>HHHHHHGSERTGTQPLGVQGLTEEQRMMIRELMDAQMKTFDTTFSHFKNFRLPGVLSSGCELPESLQAPSREEAAKWSQVRKDLCSLKVSLQLRGEDGSVWNYKPPADSGGKEIFSLLPHMADMSTYMFKGIISFAKVISYFRDLPIEDQISLLKGAAFELCQLRFNTVFNAETGTWECGRLSYCLEDTAGGFQQLLLEPMLKFHYMLKKLQLHEEEYVLMQAISLFSPDRPGVLQHRVVDQLQEQFAITLKSYIECNRPQPAHRFLFLKIMAMLTELRSINAQHTQRLLRIQDIHPFATPLMQELFGITGSSGGSGGSSHSSLTERHKILHRLLQEGSPSDITTLSVEPD[2x]

PXR is a nuclear receptor that can be activated by diverse compounds to elevate metabolism, negatively impacting drug efficacy and safety. As a xenobiotic sensor, PXR is activated by structurally diverse compounds and plays a major role in drug metabolism and drug-drug interactions by regulating transcription of genes encoding drug metabolizing enzymes, drug conjugating enzymes, and drug transporters. Here, we report structurally related PXR-selective agonists and antagonists and their corresponding co-crystal structures to describe mechanisms of antagonism and selectivity. Structural and computational approaches show that antagonists induce PXR conformational changes incompatible with transcriptional coactivator recruitment.

It should be noted that SJPYT-278 is a racemic mixture, where the (S) and (R) enantiomers were individually synthesized as SJPYT-312 and SJPYT-313, respectively. The electron density in PXR LBD complexed with the racemic SJPYT-278 mixture indicates the presence of both (R) and (S) enantiomers, likely because they have similar PXR LBD binding potency. The SJPYT-312 complex allowed visualization specifically of the (S) enantiomer. Agonistic and antagonistic activities were evaluated using a luciferase reporter under the control of a PXR-responsive CYP3A4 promoter, and as predicted, analogs with the 4-methoxy (SJPYT-326 and SJPYT-328) are agonists, and all compounds lacking the 4-methoxy (SJPYT-278, SJPYT-312, SJPYT-313, SJPYT-327, SJPYT-330, and SJPYT-331) are antagonists. Like SJPYT-310, region B of all analogs engages both the π-trap and the leucine cage, and the triazole moiety is hydrogen bonded with Q285. Like SJPYT-310, all compounds reposition F251 and the α12 residues L428 and F429. The antagonists SJPYT-312, SJPYT-331, and SJPYT-278 lack the region A 4-methoxy group and cannot effectively engage the α12 cleft. Furthermore, all antagonists consistently lose PXR L428 contact with the SRC-1 LXXLL residue L690, while the interaction is maintained by agonists. Therefore, we performed MD simulations of PXR LBD bound to agonists (SJPYT-326 and SJPYT-328) or antagonists (SJPYT-312 and SJPYT-331). While α12 of agonist-bound PXR LBD remains in the crystallographically determined inward active conformation, α12 of antagonist-bound PXR LBD moves outward to a position overlapping with the SRC-1 peptide binding site.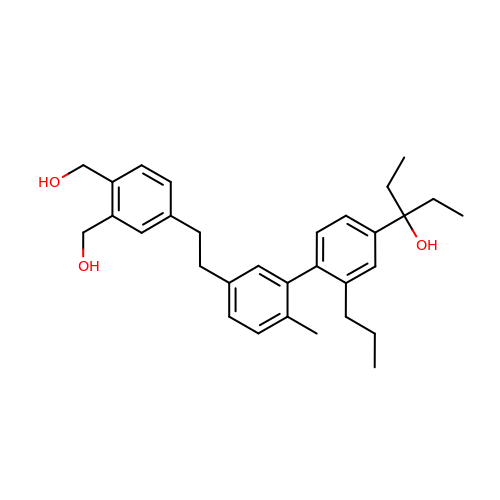3-(5'-{2-[3,4-bis(hydroxymethyl)phenyl]ethyl}-2'-methyl-2-propylbiphenyl-4-yl)pentan-3-ol | C31 H40 O3 | ONKMRBXENJVARV-UHFFFAOYSA-N> HMS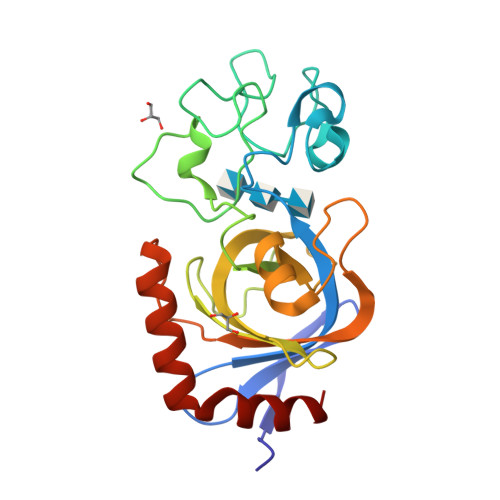ELSEIDSVAGVTIYSVDGEPKSFVYKAGFAIDADGAPNAYAPNNGGTDFTANGGDDQGGDWWGGPVDAEGYPIKQKIFDPFPGYYVSATAHFNPAYSEDSPYRYIDSNSIPFIVLPGNHSNGAKLGDVALVYNEKTGDNCYAIYGDVGPSSKIGQGSVRLAQALKIDDNPKAGGTESRIVVTLVFPGSVGKWETPKRWFSHANQLTKAWGGLSRLKTLSDQL> HHHHHHAPAFRYTRSQSFDIFDINQKCFVLESPTQLVALHLQGPSSSQKVRL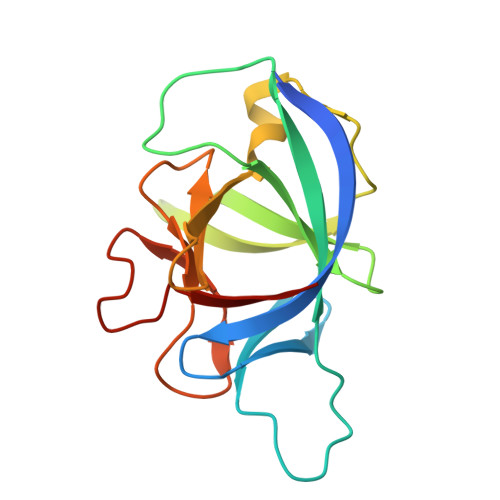NIALYRPRGPRGSAGTGQMPVALGIKGYKLYMSCVMSGTEPTLQLEEADVMRDIDSVELTRFIFYRLDSPTKGTTRFESAAFPGWFICTSLQPRQPVGITNQPDQVNIATYKLSGR> MNARKAPEFPAWPQYDDAERNGLVRALEQGQWWRMGGDEVNSFEREFAAHHGAAHALAVTNGTHALELALQVMGVGPGTEVIVPAFTFISSSQAAQRLGAVTVPVDVDAATYNLDPEAVAAAVTPRTKVIMPVHMAGLMADMDALAKISADTGVPLLQDAAHAHGARWQGKRVGELDSIATFSFQNGKLMTAGEGGAVVFPDGETEKYETAFLRHSCGRPRDDRRYFHKIAGSNMRLNEFSASVLRAQLARLDEQIAVRDERWTLLSRLLGAIDGVVPQGG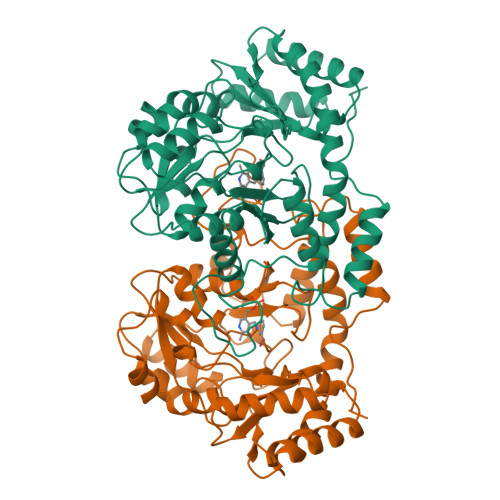DVRADRNSHYMAMFRIPGLTEERRNALVDRLVEAGLPAFAAFRAIYRTDAFWELGAPDESVDAIARRCPNTDAISSDCVWLHHRVLLAGEPELHATAEIIADAVGRA>MQVMASPPCTTEELSPPPGGSLVEYSGGSLRVPDNPVVAFIRGDGVGPEVVESALKVVDAAVKKVYGGSRRIVWWELLAGHLAREKCGELLPKATLEGIRLARVALKGPLETPVGTGYRSLNVAIRQALDLYANIRPVRYYGQPAPHKYADRVDMVIFRENTEDVYAGIEWPHDSPEAARIRRFLAEEFGISIREDAGIGVKPISRFATRRLMERALEWALRNGNTVVTIMHKGNIMKYTEGAFMRWAYEVALEKFREHVV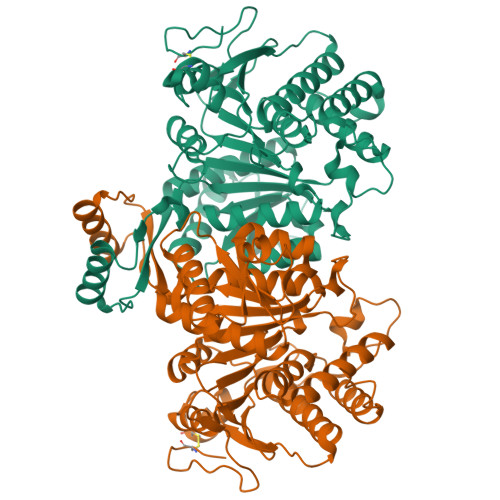TEQEVQEKYGGVRPEGKILVNDRIADNMLQQIITRPWDYQVIVAPNLNGDYISDAASALVGGIGMAAGMNMGDGIAVAEPVHGTAPKYAGKDLINPSAEILSASLLIGEFMGWREVKSIVEYAIRKAVQSKKVTQDLARHMPGVQPLRTSEYTETLIAYIDEADLNEVLAGKRG[2x]>[2x]MKKLGTLLVLFLSAIILVACASGKKDTTSGQKLKVVATNSIIADITKNIAGDKIDLHSIVPIGQDPHEYEPLPEDVKKTSEADLIFYNGINLETGGNAWFTKLVENAKKTENKDYFAVSDGVDVIYLEGQNEKGKEDPHAWLNLENGIIFAKNIAKQLSAKDPNNKEFYEKNLKEYTDKLDKLDKESKDKFNKIPAEKKLIVTSEGAFKYFSKAYGVPSAYIWEINTEEEGTPEQIKTLVEKLRQTKVPSLFVESSVDDRPMKTVSQDTNIPIYAQIFTDSIAEQGKEGDSYYSMMKYNLDKIAEGLAKGNLYF

The pneumococcus acquires Mn2+ via the PsaBCA permease, which comprises the ATP-binding cassette (ABC) transporter, PsaBC, and a cell-surface solute-binding protein (SBP), PsaA. Similar to other ABC permeases, the SBP PsaA defines the specificity of the uptake pathway. However, our recent studies showed that the functional specificity of the Psa permease in Mn2+ acquisition arose not from the specificity of Mn2+ binding by PsaA, but instead resulted from the concerted action of protein metal ion coordination chemistry and structural rearrangements that prevented release of other divalent transition metal ions, such as Zn2+, into the permease, despite their ability to bind to PsaA8. PsaA uses a ‘spring-hammer’-like mechanism for metal ion binding, in which the dynamics of the metal ion-loaded protein are dictated by a combination of metal ion geometry and the distortion of a helix linking the N- and C-terminal lobes of the protein.

Here the interaction of Cd2+ with PsaA was analysed by determining the structure of wild-type PsaA with Cd2+ at 2.0 Å resolution. The PsaA–Cd2+ complex revealed that Cd2+ was coordinated by the metal-binding site residues His67, His139, Glu205 and Asp280 in a structure that was highly similar (root-mean-square deviation (RMSD)<0.3 Å over 242 Cα atoms) to our previously reported Mn2+- and Zn2+-bound structures. Nevertheless, small re-orientations of the side chains of the metal-coordinating residues allowed the bulkier Cd2+ ion (ionic radius of 95 pm for Cd2+ versus 84 pm for Mn2+) to be accommodated into the protein–metal-binding site. In the PsaA–Cd2+ structure, the distances between metal-coordinating atoms and the metal ion were increased by ~0.2 Å compared with those for PsaA-Zn2+. Accordingly, the coordination geometry in the PsaA–Cd2+ structure is an intermediate between a square-pyramid and trigonal-bipyramid (n=5), in contrast to the 4- and 6-coordinate sites observed for the Zn2+- and Mn2+-bound PsaA structures, respectively. We then assessed the distortion of the linking helix by monitoring the number of disrupted backbone hydrogen bonds in its flexible region (residues 184–194) in wild-type PsaA–Cd2+. Both the hinge-bending angle between the N- and C-terminal lobes and the number of main-chain hydrogen bonds disrupted in the residue range 184–194 corresponded more closely to the Mn2+-bound structure than to the ‘locked’ Zn2+-structure. However, the larger ionic radius and ‘strained’ coordination of the Cd2+ ion at the metal-binding site, similar to Mn2+, resulted in an easily destabilized metal–protein complex, such that PsaA was incapable of preventing release of Cd2+ ions into the permease. In PsaA, the regulatory mechanisms that have evolved to prevent mistranslocation of Zn2+ ions are not capable of preventing the translocation of Cd2+ ions.>GFFSFIGEAFQGAGDMWRAYTDMKEAGWKDGDKYFHARGNYDAAQRGPGGVWAAEKISDARESFQ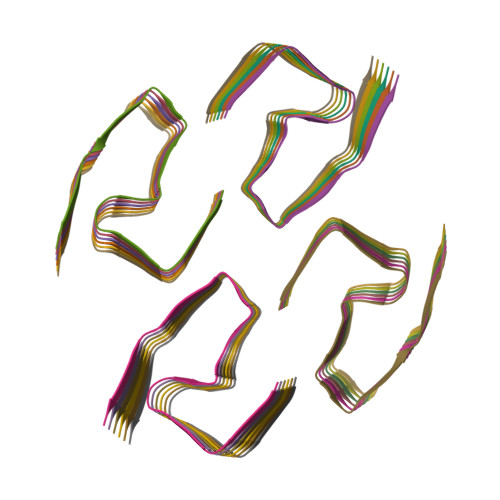EFFGRGHEDTMADQEANRHGRSGKDPNYYRPPGLPAKY[24x]>GSYAEGQRKRRNTIHEFKKSAKTTLIKIDPALKIKTKKVNTADQCANRCTRNKGLPFTCKAFVFDKARKQCLWFPFNS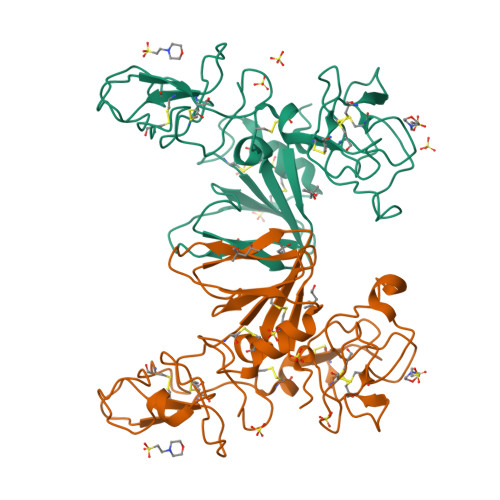MSSGVKKEFGHEFDLYENKDYIRNCIIGKGRSYKGTVSITKSDIKCQPWSSMIPHEHSFLPSSYRGKDLQENYCRNPRGEEGGPWCFTSNPEVRYEVCDIPQCSEVECMTSNGESYRGLMDHTESGKICQRWDHQTPHRHKFLPERYPDKGFDDNYCRNPDGQPRPWCYTLDPHTRWEYCKIKTCK[2x]> MRGSHHHHHHGSMSQPDATPFDYILSGGTVIDGTNAPGRLADVGVRGDRIAAVGDLSASSARRRIDVAGKVVSPGFIDSHTHDDNYLLKHRDMTPKISQGVTTVVTGNCGISLAPLAHANPPAPLDLLDEGGSFRFARFSDYLEALRAAPPAVNAACMVGHSTLRAAVMPDLRREATADEIQAMQALADDALASGAIGISTGAFYPPAAHASTEEIIEVCRPLITHGGVYATHMRDEGEHIVQALEETFRIGRELDVPVVISHHKVMGKLNFGRSKETLALIEAAMASQDVSLDAYPYVAGSTMLKQDRVLLAGRTLITWCKPYPELSGRDLEEIAAERGKSKYDVVPELQPAGAIYFMMDEPDVQRILAFGPTMIGSAGLPHDERPHPRLWGTFPRVLGHYSRDLGLFPLETAVWKMTGLTAAKFGLAERGQVQPGYYADLVVFDPATVADSATFEHPTERAAGIHSVYVNGAAVWEDQSFTGQHAG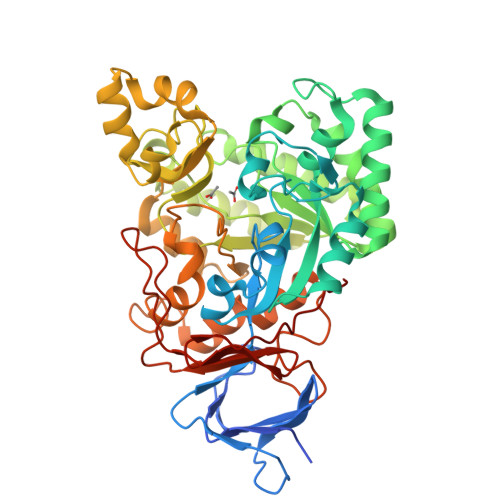RVLNRAGA> MNPIQKAWLKILEPVSYVINEKMAKRTGIIGKLGRFFAIGPREYGVHPINRMFIFMNRKYMAFQAVALHRYSFVKSLTHNGFHMLRVFRHFAFVLPATVLAGLGLFVYW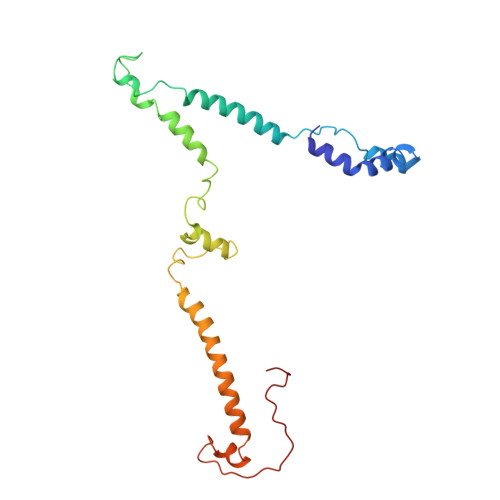GDDNKCYSPDRFPYLKKRAGDMALPLNSLNQRTSAHYIEINAIYGAEMMKRYHKVWENIIEERSKATDQEKKTRYAHPSYQYSPLPVVSIPNVLNPLNLQ>GSKDKKEAGADSKTIKLWVPTGSKKSYADTIAKFEKDSGYTVKVVESEDPKAQEKIKKDASTAADVFSLPHDQLGQLVESGTIQEVPEKYNKEIAATSTDQALIGAQYKGKTYAFPFGIESQVLFYNKSKLAAEDVTSYDTITTKATFGGTFKQANSYATGPLFMSVGNTLFGENGEDVKGTNWGNEKGAAVLKWIADQASNKGFVSLDANNVISKFGDGSVASFESGPWDYEAAQKAIGKENLGVAIYPKVTIGGETVQQKAFLGVKLYAVNQAPAKGDTKRIAASYKLASYLTNAESQENQFKTRNIVPANKEVQSSEAVQSNELAKTVITMGSSSDYTVVMPKLSQMGTFWTESAAILSDAFNGKIKESDYLTKLQQFDKDIAATK[2x]

SPs0871 is a maltodextrin-binding protein that is part of the maltodextrin transport system. Shelburne et al. previously showed that the knockout of the maltodextrin-binding protein gene did not suppress streptococcal growth in a nutrient-rich medium and that the protein played an essential role in bacterial growth in human saliva. Among the virulence factors in GAS that can be targeted, proteins involved in complex carbohydrate catabolism have been implicated in pathogen infectivity. To develop novel treatment methods that circumvent the generation of antibiotic resistance, we used virtual screening followed by several biophysical-based screening methods to identify antibacterial compounds that target SPs0871, which is a maltodextrin-binding protein that is involved in carbohydrate catabolism in GAS.

The crystal structure of SPs0871 in the absence of a ligand was determined at 2.20 Å. Three aromatic residues critical for ligand binding (Y184, W256, and W380) lined one side of the binding pocket, similar to the structure of other maltodextrin-binding proteins. The 6 of 16 residues in MalE1 that were identified in previous studies as being involved in ligand interactions are conserved in SPs0871. Given that other maltodextrin-binding proteins have been reported to adopt a closed conformation upon sugar binding, SPs0871 is likely to undergo a similar conformational change. Maltodextrin-binding proteins are thought to exist in the unbound conformation without ligands, and ligand binding drives the protein into the sugar-bound form. We first performed virtual screening for the two-state conformation of SPs0871. Using both conformations allowed us to assess whether potential ligands induce conformational changes in SPs0871 upon binding. Virtual screening with the two conformations followed by in vitro screening yielded a hit compound (95,186) that competed with the ligand and was derived from the hit library for the unbound form. Therefore, it is likely that 95,186 favorably binds to the unbound form. When we performed additional docking calculations using the Glide docking program (Schrodinger, New York, NY, USA) to identify hotspot residues for the compound binding, E146 and K294 were predicted to form hydrogen bonds and W256 was predicted to form van der Waals interactions during compound binding.2'-(L-NORVALYL)AMINO-2'-DEOXYADENOSINE 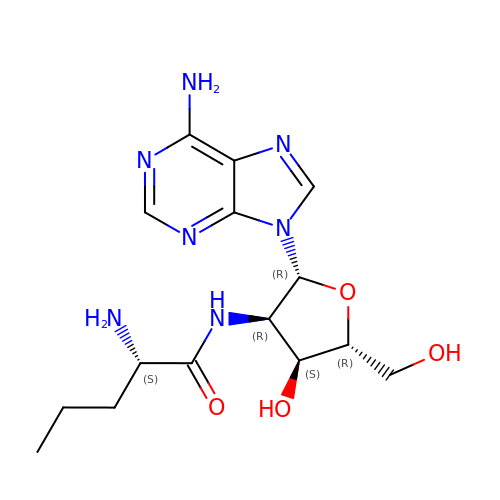| C15 H23 N7 O4 | NWKNSTYARDJRIZ-IEUWZBGXSA-N Cd2+-binding aptamers have been extensively utilized in the development of Cd2+-detecting devices; however, the underlying mechanisms remain elusive. This study reports four Cd2+-bound DNA aptamer structures, representing the only Cd2+-specific aptamer structures available to date. In all the structures, the Cd2+-binding loop (CBL-loop) adopts a compact, double-twisted conformation and the Cd2+ ion is mainly coordinated with the G9, C12 and G16 nucleotides. Other nucleotides of the loop and the G8–C18 pair of the stem also affect the Cd2+ binding, via proper folding and/or stabilizing the conformation of the CBL-loop.

The sequence of DNA1 was derived from the Cd-2-1 aptamer discovered by Wang and coworkers. DNA1 is composed of 25 nt; G1A2C3G4A5C6G7G8 at the 5′-end and C18C19G20T21T22G23T24C25 at the 3′-end are complementary to each other. The DNA1–Cd2+ complex structure was refined at atomic resolution (2.1 Å) with final Rwork and Rfree values of 23.2% and 27.4%, respectively. The structure belongs to the C2 space group, containing three DNA1–Cd2+ complexes (complexes A, B and C) per asymmetric unit. Figure 1B depicts that each DNA1 molecule can be divided into two regions, namely the stem region and the CBL-loop region, which is formed by G9T10T11C12A13C14A15G16T17 in the middle of DNA1. The root-mean-square deviation (RMSD) value between the CBL-loops of complexes A and C is 0.50 Å, and is only 0.35 Å between complexes A and B. The CBL-loop adopts one double-twisted conformation with a sharp turn at both T10 and T17 sites. The Cd2+ ion mainly coordinates with the N7 atom of G9, the N3 atom of C12 and the N7 atom of G16. Moreover, it also coordinates with two water molecules, which further stabilizes the conformation of the Cd2+ ion. The clear electron density maps support that the G4 and T22 nucleotides are well ordered and form one G–T wobble pair in the native DNA1–Cd2+ complex structure. The native DNA1 could bind very tightly with Cd2+ ions, and the value of the equilibrium dissociation constant (KD) is 0.340 ± 0.017 μM.

>[3x]GACGACGGGTTCACAGTCCGTTGTC> MFRTAYKTMNQSMVQKFIAGGVGVTGLTASYLLYQDSMTADAMTAAEHGLHPPAYNWPHNGMFETFDHASIRRGFQVYREVCAACHSLDRIAWRNLVGVSHTTSEAKAMAEELEYDDEPDDEGKPRKRPGKLADYIPGPYENEQAARAANQGAYPPDLSLIVKARHGGSDYIFSLLTGYPDEPPAGVVLPEGSNYNPYFPGGAIAMGRVLFDDLVEYEDGTPATTSQMAKDV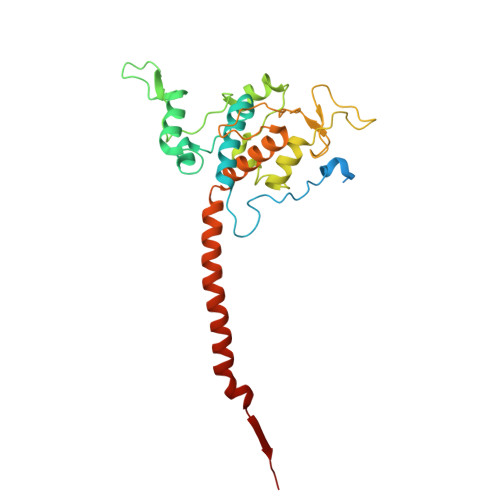STFLNWASEPEHDDRKKWGLKALVVLSSLYLLSIWVKRFKWTPIKNRKFRFDPPKK>GSHMGNRTFSYTLEDHTKQAFGIMNELRLSQQLCDVTLQVKYQDAPAAQFMAHKVVLASSSPVFKAMFTNGLREQGMEVVSIEGIHPKVMERLIEFAYTASISMGEKCVLHVMN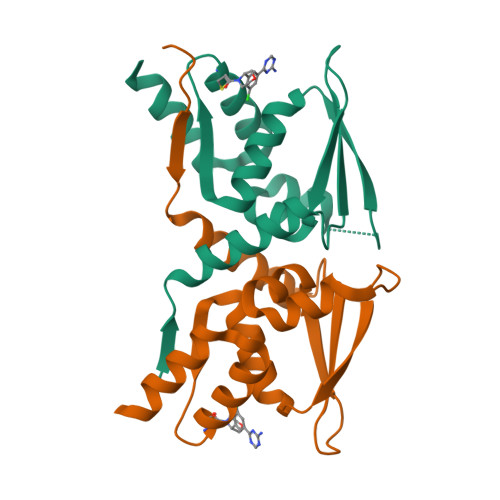GAVMYQIDSVVRACADFLVQQLD[2x]4-[5-(2-chloro-6-fluoroanilino)-6-methyl-1H-pyrazolo[3,4-b]pyridin-1-yl]-N-(oxetan-3-yl)thiophene-2-carboxamide | C21 H17 Cl F N5 O2 S | 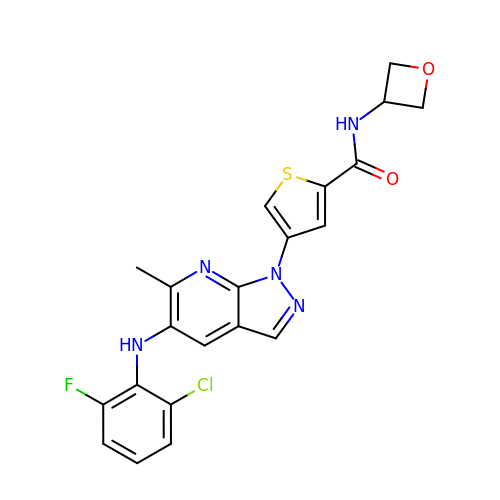KDMADGZAPDHVHE-UHFFFAOYSA-N> FKVATPYSLYVCPEGQNVTLTCRLLGPVDKGHDVTFYKTWYRSSRGEVQTCSERRPIRNLTFQDLHLHHGGHQAANTSHDLAQRHGLESASDHHGNFSITMRNLTLLDSGLYCCLVVEIRHHHSEHR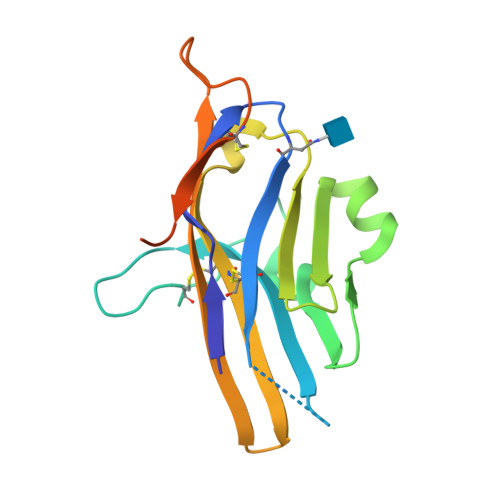VHGAMELQVQTGKDAPSNCVVYPSSSQESENITAVKLQAGFHHHHHH>DTKEQRILRYVQQNAKPGDPQSVLEAIDTYCTQKEWAMNVGDAKGQIMDAVIREYSPSLVLELGAYCGYSAVRMARLLQPGARLLTMEINPDCAAITQQMLNFAGLQDKVTILNGASQDLIPQLKKKYDVDTLDMVFLDHWKDRYLPDTLLLEECGLLRK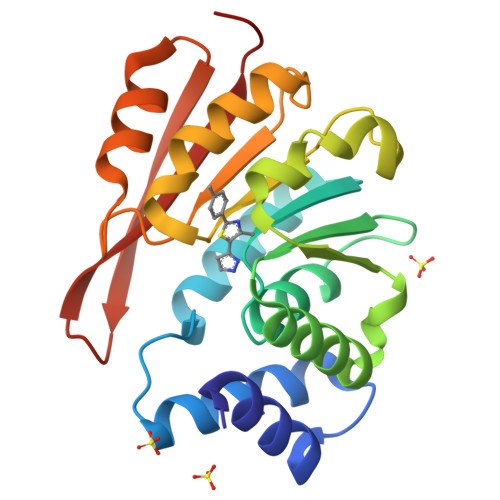GTVLLADNVIVPGTPDFLAYVRGSSSFECTHYSSYLEYMKVVDGLEKAIYQGPS[2x]>[2x]MSEKDEYQFQHQGAVELLVFNFLLILTILTIWLFKNHRFRFLHETGGAMVYGLIMGLILRYATAPTDIESGTVYDCGKLAFSPSTLLINITDQVYEYKYKREISQHNINPHLGNAILEKMTFDPEIFFNVLLPPIIFHAGYSLKKRHFFQNLGSILTYAFLGTAISCIVIGLIMYGFVKAMVYAGQLKNGDFHFTDCLFFGSLMSATDPVTVLAIFHELHVDPDLYTLLFGESVLNDAVAIVLTYSISIYSPKENPNAFDAAAFFQSVGNFLGIFAGSFAMGSAYAVVTALLTKFTKLCEFPMLET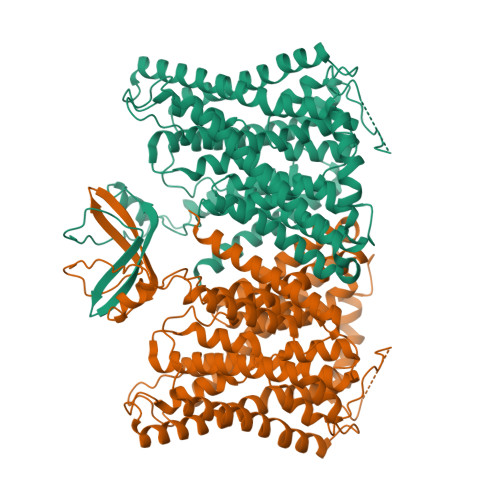GLFFLLSWSAFLSAEAAGLTGIVAVLFCGVTQAHYTYNNLSLDSKMRTKQLFEFMNFLAENVIFCYMGLALFTFQNHIFNALFILGAFLAIFVARACNIYPLSFLLNLGRKHKIPWNFQHMMMFSGLRGAIAFALAIRDTESQPKQMMFSTTLLLVFFTVWVFGGGTTPMLTWLQIRVGVDLDEDLKERPSSHQEANNLEKSTTKTESAWLFRMWYGFDHKYLKPILTHSGPPLTTTLPEWCGPISRLLTSPQAYGEQLKEGENLYFQ>GPMGQNIPIKRINVPEIGIATELSHGVVQVQFYDGSVVSVIPSMQGGGITYTQPNGTSTH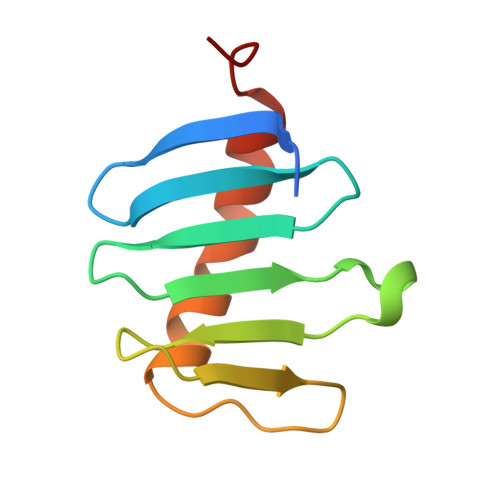FGKGDDLPFPVRDRVGQIPNIQLKLKTAPLLGS[2x]> GHMSFETRFEKMDNLLRDPKSEVNSDCLLDGLDALVYDLDFPALRKNKNIDNFLSRYKDTINKIRDLRMKAEDYEVVKVIGRGAFGEVQLVRHKSTRKVYAMKLLSKFEMIKRSDSAFFWEERDIMAFANSPWVVQLFYAFQDDRYLYMVMEYMPGGDLVNLMSNYDVPEKWARFYTAEVVLALDAIHSMGFIHRDVKPDNMLLDKSGHLKLADFGTCMKMNKEGMVRCDTAVGTPDYISPEVLKSQGGDGYYGRECDWWSVGVFLYEMLVGDTPFYADSLVGTYSKIMNHKNSLTFPDDNDISKEAKNLICAFLT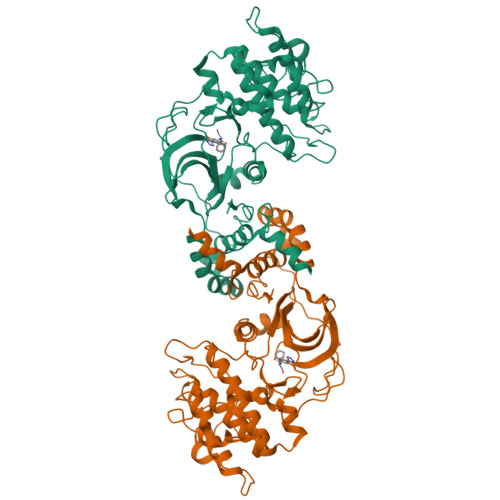DREVRLGRNGVEEIKRHLFFKNDQWAWETLRDTVAPVVPDLSSDIDTSNFDDLEEDKGEEETFPIPKAFVGNQLPFVGFTYYSNRRYLSSANPNDNR> ETGAPSPGLGPGPECFTANGADYRGTQNWTALQGGKPCLFWNETFQHPYNTLKYPNGEGGLGEHNYCRNPDGDVSPWCYVAEHEDGVYWKYCEIPACQMPGNLGCYKDHGNPPPLTGTSKTSNKLTIQTCISFCRSQRFKFAGMESGYACFCGNNPDY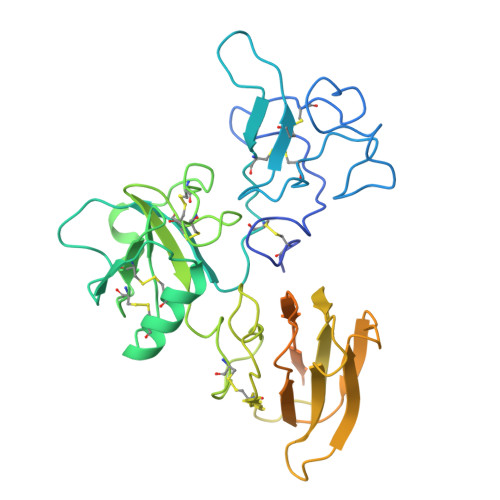WKYGEAASTECNSVCFGDHTQPCGGDGRIILFDTLVGACGGNYSAMSSVVYSPDFPDTYATGRVCYWTIRVPGASHIHFSFPLFDIRDSADMVELLDGYTHRVLARFHGRSRPPLSFNVSLDFVILYFFSDRINQAQGFAVLYQAVKEEGSENLYFQGGSLPQERPAVNQTVAEVITEQANLSVSAARSSKVLYVITTSPSHPPQTVPGTHHHHHHHHHH Here we demonstrate that HSL1 binds IDA/IDL peptides with high, and CLE peptides with lower affinity, respectively. Ligand sensing capability and receptor activation of HSL1 require a SERK co-receptor kinase. Crystal structures with IDA/IDLs or with CLE9 reveal that HSL1-SERK1 complex recognizes the entire IDA/IDL signaling peptide, while only parts of CLE9 are bound to the receptor. Our work reveals that HSL1 is a receptor for IDA/IDL signaling peptides.

The vastly different binding affinities between IDA/IDLs vs. CLE9 to HSL1 prompted us to determine co-crystal structures of four HSL1-IDA/IDL-SERK1 ternary complexes with: IDA, IDL1, IDL2, and IDL3 (at 2.31 Å, 2.38 Å, 2.20 Å, and 2.70 Å, respectively) and the HSL1-CLE9-SERK1 complex at 2.87 Å. In the presence of the co-receptor SERK1, we did observe CLE9 binding to HSL1 with a dissociation constant of 400 nM. Structural superposition of the HSL1-IDA-SERK1 and HSL1-CLE9-SERK1 complexes revealed that both IDA and CLE9 bind to the HSL1 peptide-binding surface, however, with the CLE9 N-terminus (residues 109-112) adopting a radically different orientation compared to IDA and IDLs. While the proline-rich N-terminus of IDA/IDLs accommodate into the hydrophobic cavity of the HSL1 binding surface, the corresponding region of CLE9 is unable to bind and found shifted 10 Å away from the binding groove in our structure. The lack of receptor-peptide interaction in this region is supported by the poorly defined electron density and the high atomic displacement parameters (B-factors) that indicate high flexibility of the CLE9 N-terminus. CLE9 and IDA/IDL peptides share sequence similarities in their core regions such as the Ser in position five (Ser113 in CLE9) and the Hyp in position 7 (Hyp115 in CLE9), enabling CLE9 to bind HSL1–SERK1 with lower affinity. However, Ser65IDA, which makes direct contacts with Asp283 and Tyr308 in HSL1, is an Asn residue in CLE9 that is unable to interact with the receptor-binding surface. Replacing Asn116CLE9 to a Ser results in a 2-fold increase in binding affinity to the HSL1–SERK1 complex and to detectable binding to the isolated HSL1 ectodomain. In contrast, structural analysis of the HSL1-CLE9-SERK1 complex reveals that CLE9 is only partially recognized by HSL1, rationalizing the reduced binding affinities when compared to IDA/IDLs (20-fold reduction). Taken together, HSL1 can discriminate between IDA/IDLs and the CLE9 peptide by ‘reading’ structural differences in the N-terminal and core peptide regions.

>[4x]GSSMDNQDGFILQQVKLSLDDPDSYLSSWNSNDASPCRWSGVSCAGDFSSVTSVDLSSANLAGPFPSVICRLSNLAHLSLYNNSINSTLPLNIAACKSLQTLDLSQNLLTGELPQTLADIPTLVHLDLTGNNFSGDIPASFGKFENLEVLSLVYNLLDGTIPPFLGNISTLKMLNLSYNPFSPSRIPPEFGNLTNLEVMWLTECHLVGQIPDSLGQLSKLVDLDLALNDLVGHIPPSLGGLTNVVQIELYNNSLTGEIPPELGNLKSLRLLDASMNQLTGKIPDELCRVPLESLNLYENNLEGELPASIALSPNLYEIRIFGNRLTGGLPKDLGLNSPLRWLDVSENEFSGDLPADLCAKGELEELLIIHNSFSGVIPESLADCRSLTRIRLAYNRFSGSVPTGFWGLPHVNLLELVNNSFSGEISKSIGGASNLSLLILSNNEFTGSLPEEIGSLDNLNQLSASGNKFSGSLPDSLMSLGELGTLDLHGNQFSGELTSGIKSWKKLNELNLADNEFTGKIPDEIGSLSVLNYLDLSGNMFSGKIPVSLQSLKLNQLNLSYNRLSGDLPPSLAKDMYKNSFIGNPGLCGDIKGLCGSENEAKKRGYVLEGSENLYFQ;>[4x]GSSMASANLEGDALHTLRVTLVDPNNVLQSWDPTLVNPCTWFHVTCNNENSVIRVDLGNAELSGHLVPELGVLKNLQYLELYSNNITGPIPSNLGNLTNLVSLDLYLNSFSGPIPESLGKLSKLRFLRLNNNSLTGSIPMSLTNITTLQVLDLSNNRLSGSVPDNGSFSLFTPISFANNLDLCGPVTSHPCPLEGSLENLYFQ;>RLVPSGPNPLHN[4x]>[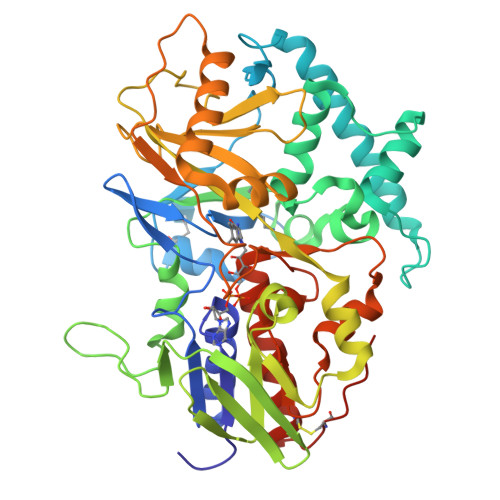2x]ATVGPRVIVVGAGMSGISAAKRLSEAGITDLLILEATDHIGGRMHKTNFAGINVELGANWVEGVNGGKMNPIWPIVNSTLKLRNFRSDFDYLAQNVYKEDGGVYDEDYVQKRIELADSVEEMGEKLSATLHASGRDDMSILAMQRLNEHQPNGPATPVDMVVDYYKFDYEFAEPPRVTSLQNTVPLATFSDFGDDVYFVADQRGYEAVVYYLAGQYLKTDDKSGKIVDPRLQLNKVVREIKYSPGGVTVKTEDNSVYSADYVMVSASLGVLQSDLIQFKPKLPTWKVRAIYQFDMAVYTMIFLKFPRKFWPEGKGREFFLYASSRRGYYGVWQEFEKQYPDANVLLVTVTDEESRRIEQQSDEQTKAEIMQVLRKMFPGKDVPDATDILVPRWWSDRFYKGTFSNWPVGVNRYEYDQLRAPVGRVYFTGEHTSEHYNGYVHGAYLSGIDSAEILINCAQKKMCKYHVQGKYDHHHHHH>FVLPATPPQLVSPRVLEVDTQGTVVCSLDGLFPVSEAQVHLALGDQRLNPTVTYGNDSFSAKASVSVTAEDEGTQRLTCAVILGNQSQETLQTVTIYSFPAPNVILTKPEVSEGTEVTVKCEAHPRAKVTLNGVPAQPLGPRAQLLLKATPEDNGRSFSCSATLEVAGQ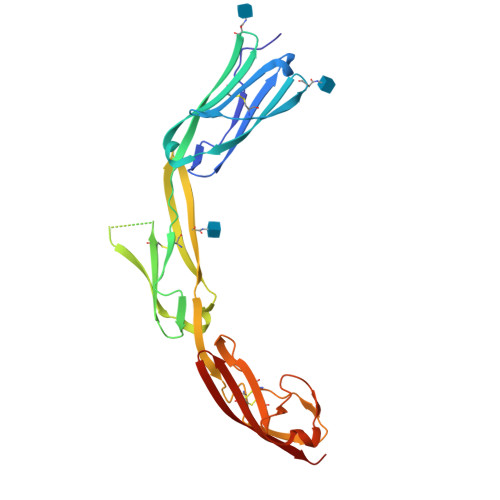LIHKNQTRELRVLYGPRLDERDCPGNWTWPENSQQTPMCQAWGNPLPELKCLKDGTFPLPIGESVTVTRDLEGTYLCRARSTQGEVTREVTVNVLSP[2x]> VKYTVENKIIAGLPKGKLKGANFVIAHETANSKSTIDNEVSYMTRNWKNAFVTHFVGGGGRVVQVANVNYVSWGAGQYANSYSYAQVELCRTSNATTFKKDYEVYCQLLVDLAKKAGIPITLDSGSKTSDKGIKSHKWVADKLGGTTHQDPYAYLSSWGISKAQFASDLAKVSGHHHHHH

PlyP100, from the GRAS Listeria phage P100, is one such endolysin that can prevent the growth of L. monocytogenes in both lab culture conditions and a miniaturized queso fresco model. Our current research focuses on the Listeria-specific N-acetylmuramoyl-l-alanine amidase PlyP100, an endolysin encoded by the bacteriophage P100, which cleaves PG at the amide linkage between the first l-alanine in the peptide chain and the lactyl group of MurNAc. After unsuccessful attempts to obtain a crystal structure of PlyP100-FL, analysis of an AlphaFold model suggested the endolysin is actually composed of three separate domains (D1, D2 and D3) separated from one another by long flexible loop regions. Our data argues that D1 is entirely responsible for catalytic activity, D3 is sufficient for cell wall binding, and D2 is necessary for full function of the enzyme, especially in food-relevant conditions.

The X-ray crystal structure of the PlyP100-D1 domain was solved to 1.80 Å resolution. The enzyme adopts a globular, mixed α/β/α fold, consisting of a central β-sheet (β1-β6) surrounded by six α-helices (α1-α6). The structure contains a single zinc ion, which is coordinated by residues His28, His137, Asp151, and His177, the latter of which results from the C-terminus of a PlyP100-D1 crystal contact. The identification of this zinc was not verified experimentally; however, its assignment is supported by analysis of the site using the Check My Metal (CMM) webserver, and is further supported by its tetrahedral coordination, favorable hydrogen bond distances, and coordination through histidine and aspartate residues, which are consistent with what is observed for catalytic zinc binding sites in proteins. During refinement, it was evident that there was clear electron density for the entire C-terminal His-tag, which was non-cleavable and therefore not removed during purification. Thus, the interaction with His177 and the aforementioned zinc ion is not present in the native enzyme and is merely an artifact of crystallization. A structural similarity search was performed using the DALI webserver, which indicated that the PlyP100-D1 domain is most structurally similar to amidases from Gram-positive bacteria. Following Cα-atom superposition, the PG was shown to be positioned in a mostly negatively charged Y-shaped crevice in PlyP100-D1, with the zinc ion situated at the branching point of the glycan and peptide chains of the PG substrate. The mutations E89A and H137A, which we propose to be important for catalytic activity, eliminated the function of PlyP100-FL against the cocktail of L. monocytogenes strains, and H149A severely impaired its function.> LFL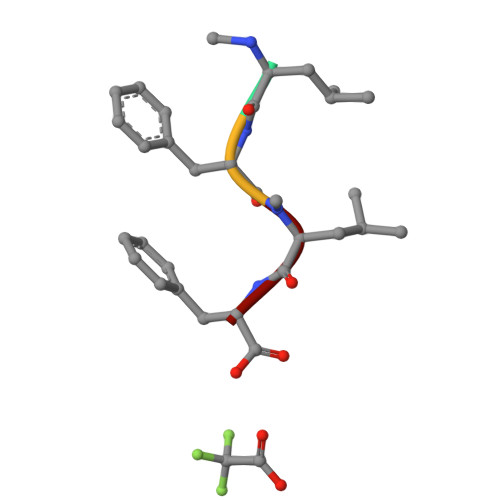F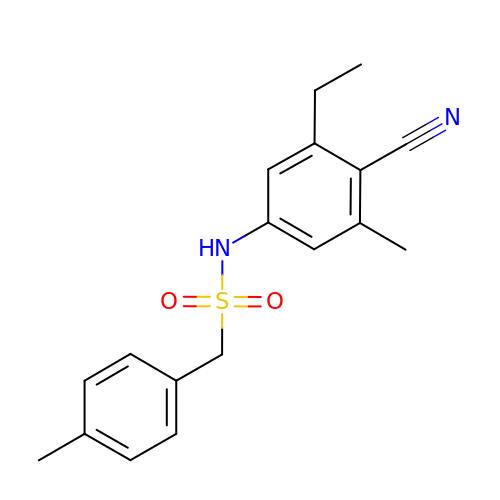N-(4-cyano-3-ethyl-5-methylphenyl)-1-(4-methylphenyl)methanesulfonamide | C18 H20 N2 O2 S | JJJGFSNVNAZOCI-UHFFFAOYSA-N>[2x]SNADNSYKMDYPEMGLCIIINNKNFHKSTGMTSRSGTDVDAANLRETFRNLKYEVRNKNDLTREEIVELMRDVSKEDHSKRSSFVCVLLSHGEEGIIFGTNGPVDLKKITN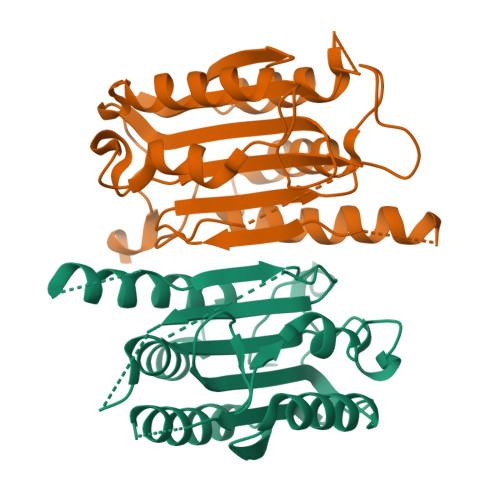FFRGDRCRSLTGKPKLFIIQAARGTELDCGIETDSGVDDDMACHKIPVEADFLYAYSTAPGYYSWRNSKDGSWFIQSLCAMLKQYADKLEFMHILTRVNRKVATEFESFSFDATFHAKKQIPCIVSMLTKELYFYH>[4x]MMIIDCHGHYTVLPKAHDEWREQQKAAFKAGQPAPPYPEISDDEIRETIEANQLRLIKERGADMTIFSPRASAMAPHVGDQSVAVPWA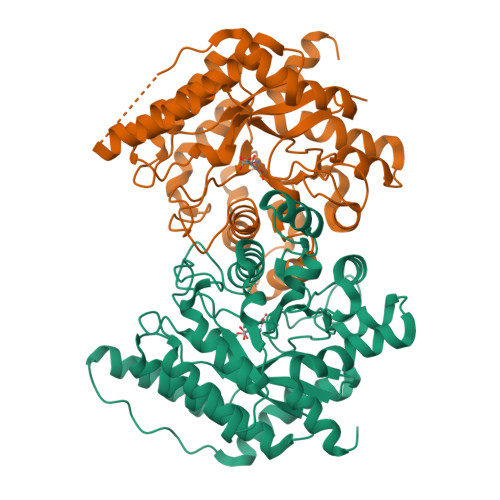QACNNLIARVVDLFPETFAGVCMLPQSPEADMTSSIAELERCVNELGFIGCNLNPDPGGGHFKHPPLTDRFWYPFYEKMVELDVPAMIHVSGSCNPAMHATGAYYLAADTIAFMQLLQGNLFADFPTLRFIIPHGGGAVPYHWGRFRGLADMLKQPSLDTLLMNNVFFDTCVYHQPGINLLADVIDNKNILFGSEMVGAVRGIDPTTGHYFDDTKRYIDALDISDQERHAIFEGNTRRVFPRLDAKLKARGL> MTQQPQAKYRHDYRAPDYQITDIDLTFDLDAQKTVVTAVSQAVRHGASDAPLRLNGEDLKLVSVHINDEPWTAWKEEEGALVISNLPERFTLKIINEISPAANTALEGLYQSGDALCTQCEAEGFRHITYYLDRPDVLARFTTKIIADKIKYPFLLSNGNRVAQGELENGRHWVQWQDPFPKPCYLFALVAGDFDVLRDTFTTRSGREVALELYVDRGNLDRAPWAMTSLKNSMKWDEERFGLEYDLDIYMIVAVDFFNMGAMENKGLNIFNSKYVLARTDTATDKDYLDIERVIGHEYFHNWTGNRVTCRDWFQLSLKEGLTVFRDQEFSSDLGSRAVNRINNVRTMRGLQFAEDASPMAHPIRPDMVIEMNNFYTLTVYEKGAEVIRMIHTLLGEENFQKGMQLYFERHDGSAATCDDFVQAMEDASNVDLSHFRRWYSQSGTPIVTVKDDYNPETEQYTLTISQRTPATPDQAEKQPLHIPFAIELYDNEGKVIPLQKGGHPVNSVLNVTQAEQTFVFDNVYFQPVPALLCEFSAPVKLEYKWSDQQLTFLMRHARNDFSRWDAAQSLLATYIKLNVARHQQGQPLSLPVHVADAFRAVLLDEKIDPALAAEILTLPSVNEMAELFD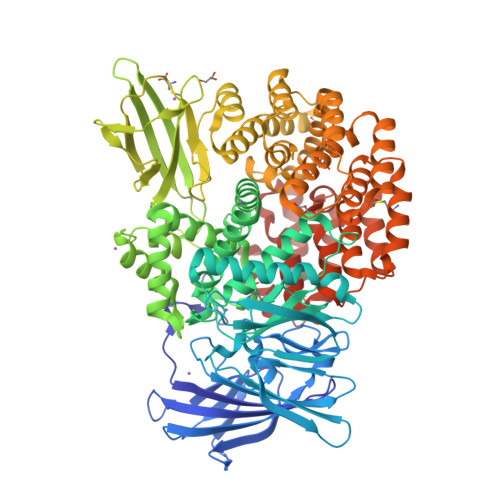IIDPIAIAEVREALTRTLATELADELLAIYNANYQSEYRVEHEDIAKRTLRNACLRFLAFGETHLADVLVSKQFHEANNMTDALAALSAAVAAQLPCRDALMQEYDDKWHQNGLVMDKWFILQATSPAANVLETVRGLLQHRSFTMSNPNRIRSLIGAFAGSNPAAFHAEDGSGYLFLVEMLTDLNSRNPQVASRLIEPLIRLKRYDAKRQEKMRAALEQLKGLENLSGDLYEKITKALA> MSAKKIVLKSSDGESFEVEEAVALESQTIA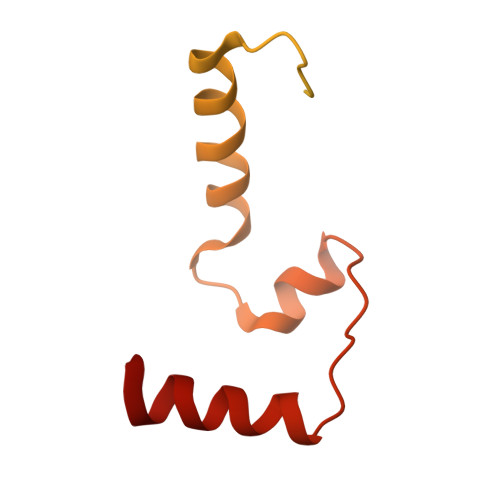HMVEDDCVDNGVPLPNVTSKILAKVIEYCKRHVEAAASKAEAVEGAATSDDDLKAWDADFMKIDQATLFELILAANYLNIKNLLDLTCQTVADMIKGKTPEEIRTTFNIKNDFTPEEEEEVRRENQWAFE> HMRKILIRGLPGDVTNQEVH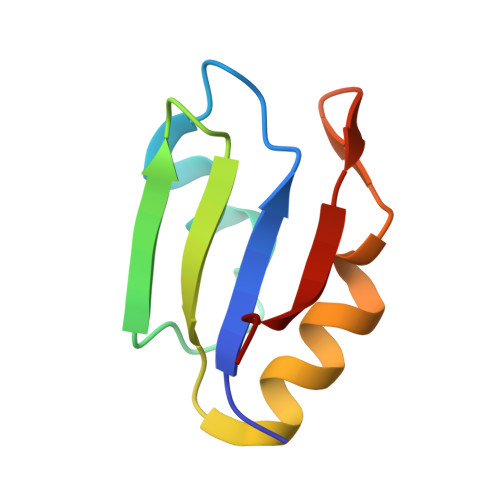DLLSDYELKYCFVDKYKGTAFVTLLNGEQAEAAINAFHQSRLRERELSVQLQPT3-chloro-N-(3-{(2S)-1-[(4-fluorophenyl)amino]-1-oxopropan-2-yl}bicyclo[1.1.1]pentan-1-yl)benzamide | C21 H20 Cl F N2 O2 | 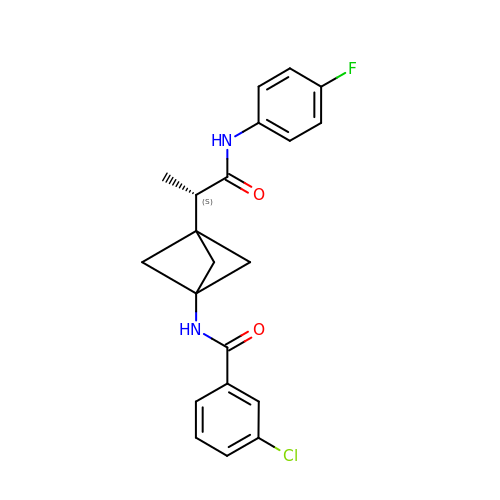ORFXTXYARYWSKK-PZVFOTJXSA-N> HHHHHAAEESPLAEIERRSGGRLGVFAIDTGSGRTLGHRADERFLMCSTFKGLLAAQILARVDSGSERLDRLVHYTEKDLIFTSPVTKANVAQGAMSIEALCRAVLVESDNTAAILLMRSAGGPAALTRFVRGLGDTVTRSDRYEPDSNRYHGVLDTTTPKAIAATAQRLLLGDV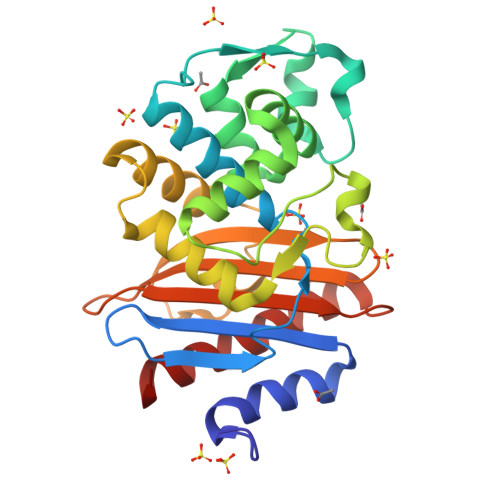LSAGSRARLERGMTDCKPGLNRIRAALPAGWLAADRPGTSVDRETNDYALVRPPGRAPLLVAVYYDAPGVSMDAREAVLREAGSAFVQWATNAG The alkaline α-galactosidase AtAkαGal3 from Arabidopsis thaliana catalyzes the hydrolysis of α-d-galactose from galacto-oligosaccharides under alkaline conditions. Here, thin-layer chromatography is used to demonstrate that AtAkαGal3 exhibits a dual function and is capable of synthesizing stachyose using raffinose, instead of galactinol, as the galactose donor. The structure of AtAkαGal3 comprises three domains: an N-terminal domain with 13 antiparallel β-strands, a catalytic domain with an (α/β)8-barrel fold and a C-terminal domain composed of β-sheets that form two Greek-key motifs. A sequence comparison of AtAkαGal3 with acidic α-galactosidases further confirmed that Asp383 and Asp447 are presumably critical residues that serve as the nucleophile and the catalytic acid/base, respectively.

Before the crystallization of wild-type AtAkαGal3, galactose was added to the protein solution via dialysis in order to obtain suitable crystals. Our first solved structure of wild-type AtAkαGal3 was thus in complex with galactose at a resolution of 2.17 Å. The crystal structure of wild-type AtAkαGal3 was first solved ab initio by the selenomethionine multi-wavelength anomalous diffraction (Se-MAD) method at a resolution of 2.8 Å and was subsequently refined to a high resolution of 2.17 Å using the native crystal with the best diffraction quality, which contains two molecules in the asymmetric unit. The structure of the AtAkαGal3–galactose complex shows that the OH group at C1, the anomeric C atom, of the galactose moiety is in a β-anomeric form and points towards the bottom side of the catalytic binding site, forming a direct hydrogen bond (distance 3.06 Å) to the nucleophile Asp383 and to the OD1 group of the acid/base catalytic residue Asp447 through a water molecule, with distances of 2.66 and 2.87 Å, respectively. Moreover, the OD1 group of Asp447 makes a strong hydrogen bond (distance 2.54 Å) to the OH2 group of the galactose. The other hydroxyl groups of the galactose are also stabilized by numerous hydrogen-bond interactions with various surrounding side chains of the residues at the −1 binding site, such as Arg443, Lys381, Asp243, Asp244 and Trp307. Furthermore, three water molecules help to stabilize the galactose moiety through water-mediated hydrogen-bonding interactions with Trp78, Lys381, Arg443, Asp447 and Asp479. The structure of wild-type AtAkαGal3 shows that the catalytic residues Asp383 and Asp447 are separated by approximately 6.7 Å, which is also generally found for the double-replacement retaining mechanism in members of clan D of the GH27 enzymes, with an average distance of 6.5 Å, and in T. maritima α-galactosidase, with a distance of 6.3 Å. Our crystal structures of wild-type AtAkαGal3 and its D383A mutant in complex with galactose and with hydrolyzed raffinose, i.e. galactose and sucrose, reveal one water molecule at the conserved position near the anomeric C atom and Asp447.

>[2x]MTIKPAVRISDGNLIIKNRTILTGVPDNVITTSASEAGPVEGVFVGAVFNKEESKHIVPIGTLRNSRFMSCFRFKLWWMAQRMGEMGRDIPYETQFLLVESNDGSHLESDGANGVECNQKVYTVFLPLIEGSFRSCLQGNVNDEVELCLESGDVDTKRSSFTHSLYIHAGTDPFQTITDAIRTVKLHLNSFRQRHEKKLPGIVDYFGWCTWDAFYQEVTQEGVEAGLKSLAAGGTPPKFVIIDDGWQSVERDATVEAGDEKKESPIFRLTGIKENEKFKKKDDPNVGIKNIVKIAKEKHGLRYVYVWHAITGYWGGVRPGEEYGSVMKYPNMSKGVVENDPTWKTDVMTLQGLGLVSPKKVYKFYNELHSYLADAGVDGVKVDVQCVLETLGGGLGGRVELTRQFHQALDSSVAKNFPDNGCIACMSHNTDALYCSKQAAVIRASDDFYPRDPVSHTIHIASVAYNSVFLGEFMQPDWDMFHSVHPAAEYHASARAISGGPLYVSDSPGKHNFELLRKLVLPDGSILRARLPGRPTRDCLFADPARDGVSLLKIWNMNKYTGVLGVYNCQGAAWSSTERKNIFHQTKTDSLTGSIRGRDVHSISEASTDPTTWNGDCAVYSQSRGELIVMPYNVSLPVSLKIREHEIFTVSPISHLVDGVSFAPIGLVNMYNSGGAIEGLRYEAEKMKVVMEVKGCGKFGSYSSVKPKRCVVESNEIAFEYDSSSGLVTFELDKMPIENKRFHLIQVEL(1~{S})-1-methyl-2,3,4,9-tetrahydro-1~{H}-pyrido[3,4-b]indole | C12 H14 N2 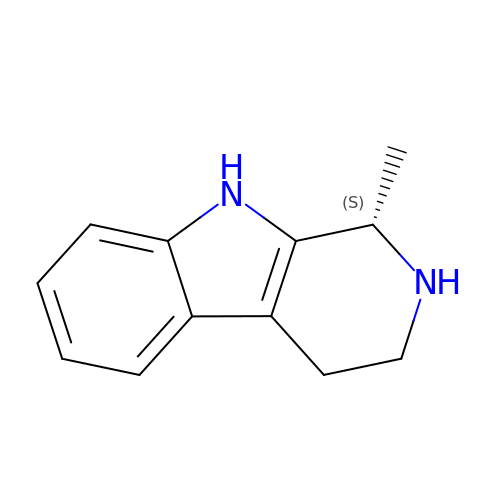| LPIJOZBIVDCQTE-QMMMGPOBSA-N E. coli aspartate aminotransferase (AAT) is a pyridoxal phosphate (PLP)-dependent enzyme that catalyses the reversible transamination of l-aspartate with α-ketoglutarate, yielding oxaloacetate and l-glutamate. During its catalytic cycle, AAT undergoes hinge movement to switch between an open conformation, in the ligand-free form, and a closed conformation upon association with substrates or inhibitors. Using our approach, we enrich the less populated but catalytically active closed conformation in order to increase catalytic efficiency (kcat/KM) with the non-native substrate l-phenylalanine, leading to altered substrate selectivity. Steady-state kinetics reveal kcat/KM increases of up to 100-fold towards this aromatic amino acid, resulting in a selectivity switch of up to 1900-fold, and structural analyses by room-temperature X-ray crystallography and multitemperature nuclear magnetic resonance (NMR) spectroscopy confirm that the conformational landscape is remodeled to favor the target state.

We collected X-ray diffraction data at room temperature (278 K) for all variants with the exception of AIFS, which could only be measured at cryogenic temperature (100 K) because we could only obtain small crystals that were not robust to radiation damage at non-cryogenic temperatures. All six enzymes yielded crystals under similar conditions, which could only be obtained in the presence of maleate, an inhibitor that stabilizes the closed conformation when bound by both WT25 and HEX14. In the inhibitor-bound state, all structures were closed as expected due to electrostatic interactions between maleate and the side chains of Arg280 and Arg374. Overlay of AAT structures (Chain A) in the presence and absence of maleate show transition from open to closed states upon inhibitor binding for WT, VFCS, and AIFS, but not for HEX, VFIT, and VFIY, which already adopt the closed conformation in the absence of bound inhibitor. Interestingly, the amplitude of the open/closed conformational transition that occurs in open variants upon maleate binding correlated with their computed ΔE values (VFCS < WT < AIFS), suggesting that this metric can be used to fine-tune this enzyme conformational landscape. Furthermore, DynDom analyses of all variants confirmed that only WT, VFCS, and AIFS undergo hinge motion upon maleate binding, which rotates the moving domain relative to the fixed domain by 4.6, 2.6, and 5.9 degrees, respectively. OpenLow mutants had lower KM values and were more catalytically efficient than WT with both l-phenylalanine and l-aspartate, which could be due to the fact that these mutants have ΔE values similar to the WT but stabilize both the open and closed conformations by >10 kcal mol‒1.

>MAHHHHHHVGTFENITAAPADPILGLADLFRADERPGKINLGIGAYIDETGKFPVLTSVKKAEQYLLENETTKSYLGIDGIPEFGRCTQELLFGKGSALINDKRARTAQTPGGTGALRVAADFLAKNTSVKRVWVSNPSWPNHKSVFNSAGLEVREYAYYDAENHTLDFDALINSLNEAQAGDVVLFHGCCHNPTGIDPTLEQWQTLAQLSVEKGWLPLFDFAYQGFARGLEEDAEGLRAFAAMHKELIVASSYSKNFGLYNERVGACTLVAADSETVDRAFSQMKAAIRANYSNPPAHGASVVATILSNDALRAIWEQELTDMRQRIQRMRQLFVNTLQEKGANRDFSFIIKQNGMFSFSGLTKEQVLRLREEFGVYAVASGRVNVAGMTPDNMAPLCEAIVAVL[2x]> MNAHFANEVQYDLTRDPSSPASLIHVIISSECLAAAGVPLSALMRGRPDGGAAANFRVETQTRAHATGDCTPWRSAFAAYVPADAVGALIAPVVPAHPDLLPRVPSAGGLFVSLPVACDAQGVYDPYTVAALRLAWGPWATCARVLLFSYDELVPPNTRYAADGARLMRLCRHFCRYVARLGAAAPAAATEAAAHLSMGLGESGTPTPQASSVSGGAGPAVVGTPDPPISPEEQLTAPGGDTATAEDVSITQENEEILALVQRAVQDVTRRHPVRARPKHAASGVASGLRQGALVHQAVSGGALGASDAEAVLAGLEPPGGGRFASRGGPRAAG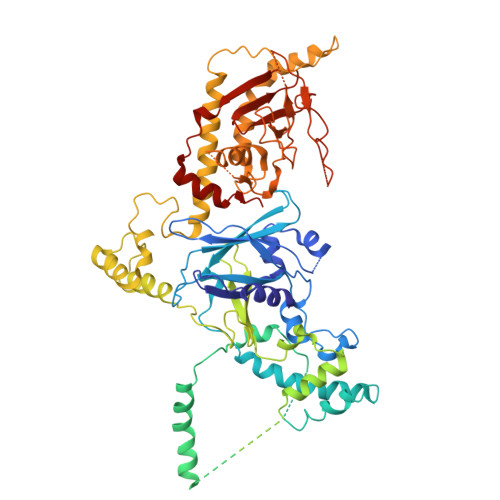EDVLNDVLTLVPGTAKPRSLVEWLDRGWEALAGGDRPDWLWSRRSISVVLRHHYGTKQRFVVVSYENSVAWGGRRARPPRLSSELATALTEACAAERVVRPHQLSPAAQTALLRRFPALEGPLRHPRPVLQPFDIAAEVAFVARIQIACLRALGHSIRAALQGGPRIFQRLRYDFGPHQSEWLGEVTRRFPVLLENLMRALEGTAPDAFFHTAYALAVLAHLGGQGGRGRRRRLVPLSDDIPARFADSDAHYAFDYYSTSGDTLRLTNRPIAVVIDGDVNGREQSKCRFMEGSPSTAPHRVCEQYLPGESYAYLCLGFNRRLCGLVVFPGGFAFTINTAAYLSLADPVARAVGLRFCRGAATGPGLVR>[2x]MNGNDPDIAGFKQQLVQMTAMRESQPPSIEIERQMFDAQHGAVPPAEGCLIEPISTGGVRGERITPKSADTSKALIYFHGGGHLFGSALSHRHLVSRLAAAAGVVAYNMEYRLAPENPYPAGLDDAE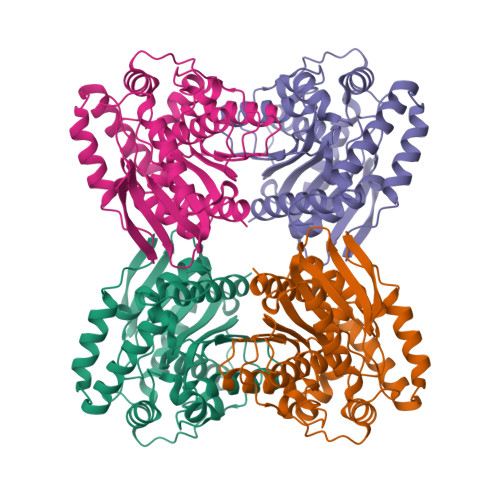QAYRFVLAQGFKPEDIIVAGESAGGNLAAALLLKLRDQDLPQPAGAYLLSPWLDMSQSGASYEARGPHDPMITHNALTGCSAAYRAGASAEDPLISPAKADLADLPSLFIQVGADEVLLSDSVEFTRRAALAGLDVRLHVWANMVHAWPLFHFALPVSGLAAIDEAGAWISRQLGGHLEHHHHHH>[5x]XGNI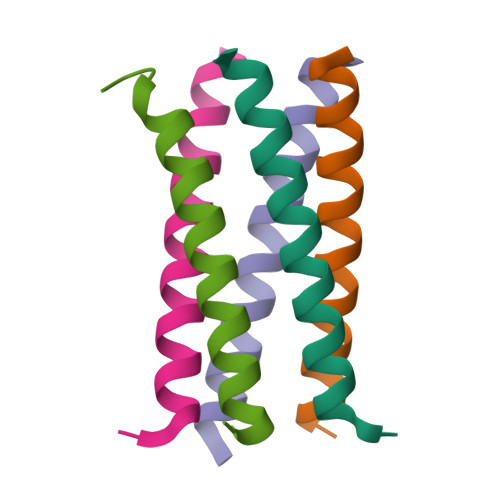LQKIENILKKIENILWKIENILQKIEG>[3x]ATPHINAEMGDFADVVLMPGDPLRAKYIAETFLEDAREVNNVRGMLGFTGTYKGRKISVMGHGMGIPSCSIYTKELITDFGVKK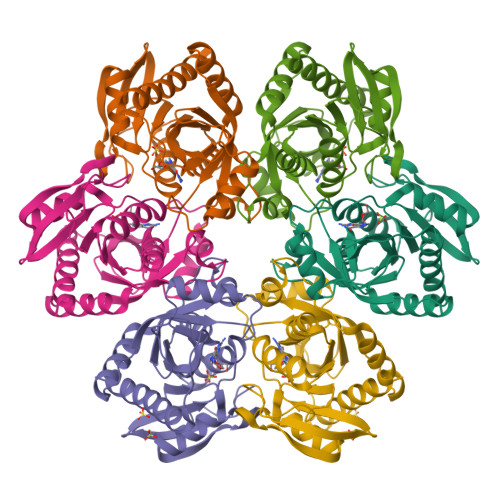IIRVGSCGAVLPHVKLRDVVIGMGACTDSKVNRIRFKDHDFAAIADFDMVRNAVDAAKALGIDARVGNLFSADLFYSPDGEMFDVMEKYGILGVEMEAAGIYGVAAEFGAKALTICTVSDHIRTHEQTTAAERQTTFNDMIKIALESVLLGDK>[5x]AMAGVFTYESEFTSVIPPPKLFKAFVLDADNLIPKIAPQAVKSAEIIEGDGGVGTIKKIHLGEGSEYSYVKHKIDGIDKDNFVYSYSIIEGDAIGD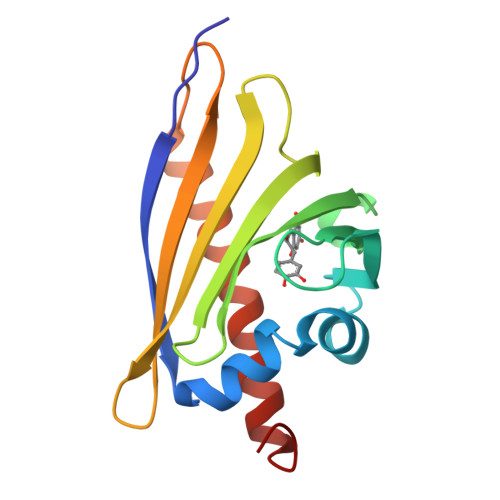KIEKISYEIKLVASGGGSIIKSTSHYHTKGEVEIKEEHVKAGKERAAGLFKIIENHLLAHPEEYN Mitochondrial proteins CHCHD10 and CHCHD2 are mutated in rare cases of heritable FTD, ALS and PD and aggregate in tissues affected by these diseases. Here, we demonstrate that the low complexity N-terminal domains of both D10 and D2, as well as the full-length proteins, can form amyloid fibrils in vitro and in vivo. Structures of D10 and D2 fibrils assembled in vitro from the low complexity N-terminal domains of each protein show that their core comprises the most highly conserved region between the two proteins. For D10 and D2, the central conserved VAV motif forms a beta-strand that is associated with the protofilament interface in all the structures we have observed, suggesting that it may be a critical element in fibril formation and may be expected to appear in ex vivo structures as well.

Using cryo-EM, we observed several distinct D10-NT fibril polymorphs (see Methods section on Cryo-EM sample preparation and data collection) and determined three different structures. Polymorph-2, solved to 2.70 Å resolution, also contains two identical symmetry-related PFs, with a fold (PF2) distinct from that found in polymorph-1 (PF1). PF2 is comprised of residues G43–G76 and exhibits four strands consisting of residues M45–A53 (similar to strand-1 in PF1), V55–V57 (similar to strand-2 in PF1), A60–V64 and L69–F73. An extensive inter-PF2 interface is comprised of strands 2–4. However, in the PF2 and PF3 D10-NT folds, some of the sequence variation sites are positioned within the PF fold, suggesting that these D10-NT folds may not be compatible with the D2 sequence. For WT D10-NT, we obtained 2D classes closely resembling those observed for WT D10-NT polymorph-2. We have provided evidence in the form of 2D classes obtained from cryo-EM datasets of independent samples that the WT D10-NT polymorph-2, the S59L D10-NT and the WT D2-NT structures we determined are reproducible and may therefore be preferred by their respective variants. The resulting structure was nearly identical to the WT D10-NT polymorph-2 structure, indicating that this mutation likely does not alter D10 fibril structure.

>MPRGSRSAASRPASRPAAPSAHPPAHPPPSAAAPAPAPSGQPGLMAQMATTAAGVAVGSAVGHVMGSALTGAFSGGSSEPSQPAVQQAPTPAAPQPLQ[18x]> GEFSTTPGGTRIIYDRKF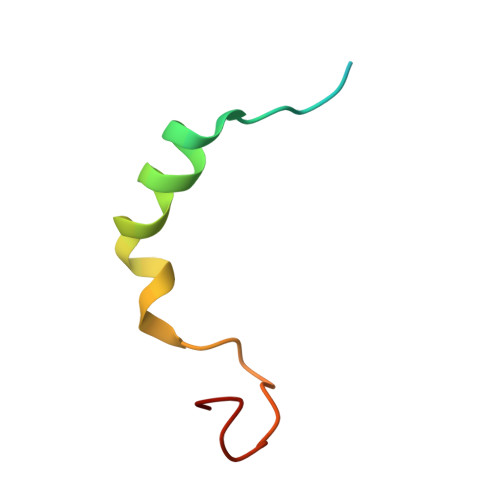LMECRNSPVTKTPPRDLPTIPGVTSP>MSRNNDINAEVVSVSPNKLKISVDDLEEFKIAEEKLGVGSYLRVSDNQDVALLAIIDNFSIEVKESQKQKYMIEASPIGLVKNGKFYRGGDSLALPPKKVEPAKLDEIISIYSDSIDINDRFTFSSLSLNTKVSVPVNGNRFFNKHIAIVGSTGSGKSHTVAKILQKAVDEKQEGYKGLNNSHIIIFDIHSEYENAFPNSNVLNVDTLTLPYWLLNGDELEELFLDTEANDHNQRNVFRQAITLNKKIHFQGDPATKEIISFHSPYYFDINEVINYINNRNNERKNKDNEHIWSDEEGNFKFDNENAHRLFKENVTPDGSSAGALNGKLLNFVDRLQSKIFDKRLDFILGEGSKS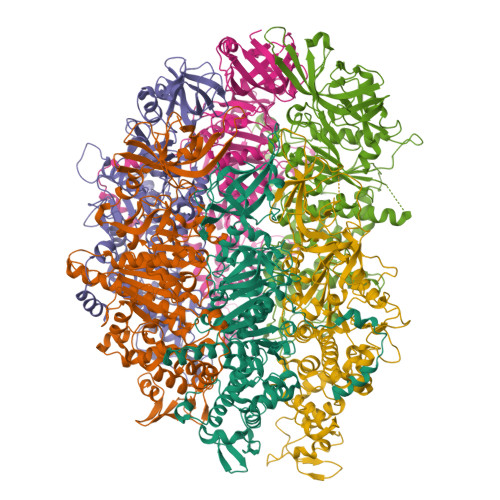VTFKETLETLISYGKDKSNITILDVSGVPFEVLSICVSLISRLIFEFGYHSKKIKRKSNENQDIPILIVYEEAHKYAPKSDLSKYRTSKEAIERIAKEGRKYGVTLLLASQRPSEISETIFSQCNTFISMRLTNPDDQNYVKRLLPDTVGDITNLLPSLKEGEALIMGDSISIPSIVKIEKCTIPPSSIDIKYLDEWRKEWVDSEFDKIIEQWSKS[6x]> SMADRGDSGDSDFVVVANRLPIDLERAPDGTTSWKRSPGGLVTALEPLLRRRRGAWIGWPGIPDSDEDPIVDGDLVLYPVRLSADDVAQYYEGFSNATLWPLYHDVIVKPIYNRQWWERYVEVNRRFAEATSRAAARGATVWVQDYQLQLVP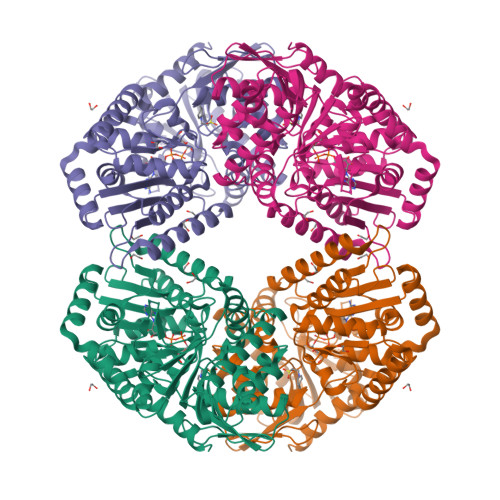KMLRELRPDLTIGFFLHIPFPPVELFMQLPWRTEITDGLLGADLVGFHLPGGAQNFLFLARRLVGANTSRASVGVRSKFGEVQIGSRTVKVGAFPISIDSADLDRQARQRSIRQRARQIRAELGNPRRILLGVDRLDYTKGIDVRLQAFAELLAEGRVNREDTVFVQLATPSRERVEAYRLLRDDIERQVGHINGEYGEVGHPVVHYLHRPVPREELIAFFVAADVMLVTPLRDGMNLVAKEYVACRSDLGGALVLSEFTGAAAELGQAYLVNPHNLDHVKDTMVAALNQTPEEGRRRMRALRRQVLAHDVDLWARSFLDALASTRTGDADAVPV> ACTKNAIAQTGFNKDKYFNGDVWYVTDYLDLEPDDVPKRYCAALAAGTASGKLKEALYHYDPKTQDTFYDVS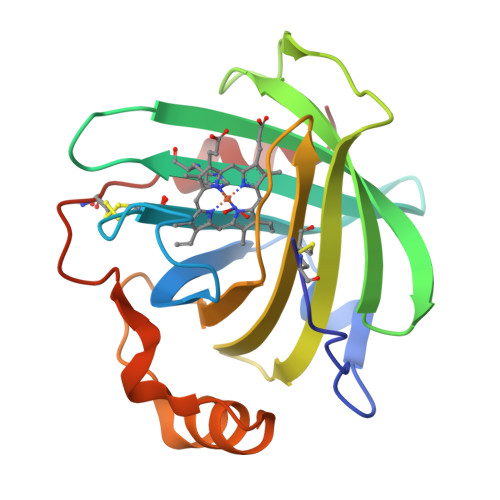ELQVESLGKYTANFKKVDKNGNVKVAVTAGNYYTFTVMYADDSSALIHTCLHKGNKDRGDLYAVLNRNKDAAAGDKVKSAVSAATLEFSKFISTKENNCAYDNDSLKSLLTK>[2x]AEQKTLHIYNWSDYIAPDTVANFEKETGIKVVYDVFDSNEVLEGKLMAGSTGFDLVVPSASFLERQLTAGVFQPLDKSKLPEWKNLDPELLKLVAKHDPDNKFAMPYMWATTGIGYNVDKVKAVLGENAPVDSWDLILKPENLEKLKSCGVSFLDAPEEVFATVLNYLGKDPNSTKADDYTGPATDLLLKLRP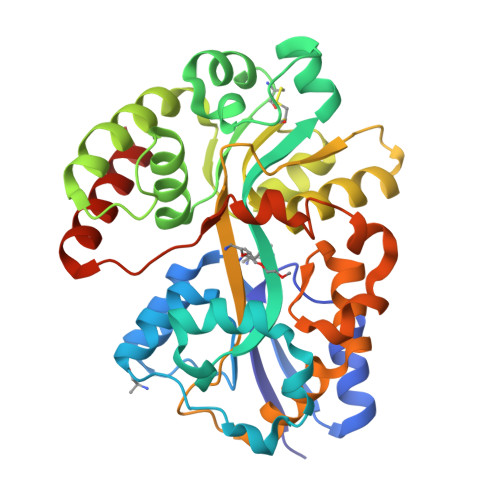NIRYFHSSQYINDLANGDICVAIGWAGDVWQASNRAKEAKNGVNVSFSIPKEGAMAFFDVFAMPADAKNKDEAYQFLNYLLRPDVVAHISDHVFYANANKAATPLVSAEVRENPGIYPPADVRAKLFTLKVQDPKIDRVRTRAWTKVKSGKLEHHHHHH>[3x]MKKIYFMLAIAGIFAGCVPSANSATKNSSANSTAPSQDVIVQKVDKDDVRDIIREEKMLAPDASETELSFTAVGEGIAPMNTVSTAQALALAKRAAITDAYRQLASKLYGVKVNGKDTVKDAMLRSSTITAQVNGLIKNASIIDENFNQGLYRVNLELKIDADKWKELFAY;>MKKILIICMLFTLSFGIERPKFEDFLAGYERNKASMLNYEGMPAFALSENLLAVLKQPNTKLNKYVKYDPFLNLYLVRTDFSLIPTPMGDEEKLTRNDWVGIWDPNKPYIGHIKYLAQNIDEKDQLDFNSKIGLLGTPCCEMMGIALNNSSFIGNRYLKHFMKYNDVYWGDIGVDFVVRENKIYVNNVRKNPQFLINDQVISVDGLPANDLRKLNEKILFADRGSTLYFQVLRDNMDLNISTEVFAKDLSKFNLPDSKPKPKITNFTSNLGLTVNTSLVVTKIDPKSKASNAGFMVGDKILRVNNIILNNFKELQNILSAGNDFSILIERKSTKLPLSNFNNELGGNANSGGDGKFQFFIRLTK[7x];> MRILFLILLSFLNAFAFELVLNTGRENNQAFAVLHASNDLEFTCQKFITEAKVHFECDIVGMVDNKLKDQSFSAFDLKFIQEAQKIKMIILPKIQARMFDTSQNIYIDKELSSSSSHKSKAFTFIFTPELAPIKDYDGLDFNINFPHESLPYVGALDLNSDPVVIPQSADINTYLRIKKEYDKANYNQVVIDAQNAINRYRGSIFTSEFILYKLRAQNKLYTQDPSMRDQQILEKMIDDAKNWTRTFTSDKNFSEVLHIMLRTYIALAQRADVEYTMSILDNEQPNNYFTQLSKLDYADYIYNLNEKEKAVNIYENTYFNTKNLDLAARAAMSLAKNLLSNEQVNKAIEYINTILKANPEYFGKDIPRSLELAKLFNQKGQFDISASIYEDAFAKMSKLDPSYEETLKDLALVLSHANRSSDAKKYLDLYMDDYLDGKYLDEIKKASDEVFFALGDNNASFLHQRYTDLMKQYANKDENIANKALDEDVALYYKEGNFSAILAYKDLIESKKIPNATQFLEKAAINDLKNAIKADNCINAANIFMRFSAYDIGQKIENKKQMLACLIRTSNVEQALDYIDKNYNEDSIFYGLQKASILFDNKQYPQVIKISKDIANSRILKSDDENFKAYYLQFLSLLRLNDYNQAIKILQILESFPMNFSMVEAYDALLSYANDHNMQTTILTYAPKAIDYQNFKGINLFSPNLEFIYLDALTKINKNEESLAVLTDL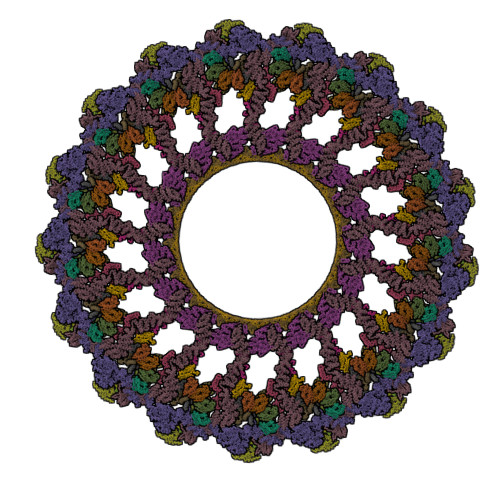LKLKLSDEDRARALYIQALTYERMQNIQAEKESLKQCLEIKSASNWQNLCKSKNQILNQ;> MAEQEDIILEKPEDGLNQPRLDESLEGFKGQEGQAPEDEEFASLPEELPQENSESGFKFTRESAPEDVSTFEEVESQEPTPWYKDRKFMSLVGLSLGIICILVFTLFYLTFSEGKIKPDIIASKPLEQPVVMPDESYKYNDMQRIDGMIQKANALYLKGEVEQALKVYEQVAVYNESLSNYNLGVSQMNENKFQEAFESFKKAIANGENQSVAAINAAVCALKLNDKEKFRYYIDLAQVYLPKEGKSKLYDYYLSLINYYKGYYPEALQMLQRTDMEPYSDVAKYLSAKIYAKMDFDSKAIQQLNSQGNFESSLSLGLLYARIGEYAKAKVALSTAMKIERDFNQSLAALTLVDIKTGNYQDMLARLQNSYDNDKDRYKILDAYKIQVRLNKDLFNIAVAQNSFSKDLLKKQKDQFDLLFYFAPYQVFDSKQAALYIKKANVTDFVDDSADAGVYLNTSKALSSTNVKIANIINYALNQKLRLANQEFQKLIKDYPEHSILHYNLALTYAQMQNYELAYKHFSSSYHLNPKNYLAGAFAMFCAKLIDIDTTKLYNEILDNIAADSNFKANMQKSMLFLVNNNYISMLPYLDETKKDTPLSLIFEAIVAKNNNLNNQVDVKIAKLRSELPEDILANILYFNSLNSNLNIKEYAQNAQIHFKNLKLDYRSVFGGPNIAREFYVNLMHIAGLLNLERQKIKELINVSGAKDEGILQTLAYLDIFAQQYEEAYALYNSLIDDYGAKDTKTLFLAAVAAIGANNPNSAIALLQLSKLTDKNNKESKAALGMLYQEVKNYEAAISQYKTLPNNFKSEFFTFDINNN;>MAKKHKCPECPAGEKWAVPYADFLSLLLALFIALWAISKTNPAKVEALKTEFVKIFDYTSTQTVKEESKTQEKYKGAAKEESDELKSLKQMTMTQQETIKRLQAALDQSDNQVALNLPSKVEFERGSAQIVSADIQDYLKRMAELTTYLPPQAKIEIRGYTDNSDSIIRSYELAYQRAENVLKYFIEGGANLKNISIKSYGLNNPINGNPQALENNRVEIYFKVDTADTSTQKSVLELINKIGTKAP[2x];>MDEELENEETKKKKGGSLVIIIVILLFVLLLSIMGVIAWLISSSSSDESEVKEAPKEEAKADKPKVSAPTQRGSDFANIGPMYPLDPFTLNLLSDSGSRYVKCTIELEQNSELLKPELDKKVPVIRDIIIRTLTAKTFEEVSTQKGKERLKDELVGKINEILTDGFIKNVYFTDFVVS[4x]>HHHHHHTSCNPSDMSHGYVTVKPRVRLHFVELGSGPAVCLCHGFPESWYSWRYQIPALAQAGYRVLA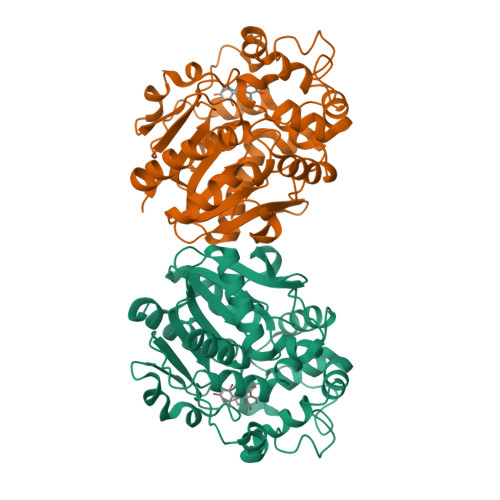MDMKGYGESSAPPEIEEYCMEVLCKEMVTFLDKLGLSQAVFIGHDWGGMLVWYMALFYPERVRAVASLNTPFIPANPNMSPLESIKANPVFDYQLYFQEPGVAEAELEQNLSRTFKSLFRASDESVLSMHKVCEAGGLFVNSPEEPSLSRMVTEEEIQFYVQQFKKSGFRGPLNWYRNMERNWKWACKSLGRKILIPALMVTAEKDFVLVPQMSQHMEDWIPHLKRGHIEDCGHWTQMDKPTEVNQILIKWLDSDARNPPVVSKM[2x]> MQTPSIIQCGLLNSFARKMTDAISDNQIIATSRFFNI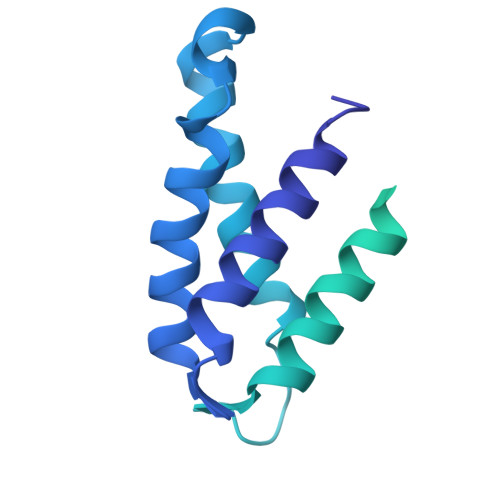ARDVADVVVSNTKLAQQYEQLSIDSLKEYLVSVAKFVAVDYSNTTSADVDDLIHKLRLFIEEECYQYNIDKEETCDGDVCVSDEYNEPAPKPKPKPKPKPAPKPKPAPKPKPAPKPAPKPAPKPAPKPAPKPAPKPAPKPAPEPAPEPAPEPAPKPAPEPAPEPAPIRPARRCDENPSNLETCCTNKALYGDFTDSSCDIVKKKTNWWLWGGIAILVIVLMIGGYFIYKRYFSAPKFENTGEFVNDMNFNNDVNFNNDVNFDNDMNYGNEGIDVSDLEILNLPVPSVSPVPSASIVPSVSPIPRGSPVPSASPIK>MRKFILSLSILLSALLVACSSRNHYGDTGSLAGLQAMADSKYTRAQKKQKMGKIREMALKETALSVGAQAGLAWRAKIIDEQLNKQARNLDAIYDFNSLVLEHNILPPVLLEGRNTLNLADAQSIRISDRTYKVAKQAHFITTPPTWRQYLWMDYVKPEAPNVTLLPKTKAEKEIWCIYTERGWKNGIDQANTILEENIARIKEDFGGMILYRKLLAMNMVSPPYVSHTDLGVTGDGSEIHIDDRVLRITALPELNVNSAEWRAAVAKDENALERFKNMEKLANQAKIVITNKSWQPIIAPVS[13x];>[26x]MNNNKIVIMFIFSALLAGCAGTMKFKKPPINNPSDDATIKLAEAAVSVSDSMLEMAKVEKVITPPSKDNTLTIPNAYNLQARASVDWSGPIEELTARIAKAAHFRFRVLGKSPSVPVLISISTKDESLAEILRDIDYQAGKKASIHVYPNSQVVELRYAKIYS;>[13x]MMKKYDQLCKYCLVIGLTFSMSCSIYAADQSDDAQQALQQLRMLQQKLSQNPSPDAQSGAGDGGDNAASDSTQQPNQSGQANAPAANQTATAGGDGQIISQDDAEVIDKKAFKDMTRNLYPLNPEQVVKLKQIYETSEYAKAATPGTPPKPTATSQFVNLSPGSTPPVIRLSQGFVSSLVFLDSTGAPWPIAAYDLGDPSSFNIQWDKTSNTLMIQATKLYNYGNLAVRLRGLNTPVMLTLIPGQKAVDYRVDLRVQGYGPNAKSMPTEEGIPPSANDLLLHVLEGVPPPGSRRLVVSGGDARAWLSNEKMYVRTNLTILSPGWLASMTSADGTHAYEMQKSPVLLVSWHGKVMQLKVEGL;>MRSLRTNYIYVLFKTTGLLFLLLLSACNRSGYIPENEVPKLPCRVDGACDATIIKMMTDLNKKGIKVASVGQNYLISIPASALFADQSPRLNWASYSLLNEIAAFLKQFRKIAITVTSYSSKYVSVKRERALTLARSRVVSEYLWSQGVDSRIIFTQGLGSDKPITSYTLGGDRSPNARVEITFRRAVA[13x];>[52x]AAAAAAAAAAAAAAAAAAAAAAAAAAAAAAAAAAAAAAAAAAAAAAAAAAAAAAAAAAAAAAAAAAAAAAAAAAAAAAAAAAAAAAAAAAAAAAAAAAAAAAAAAAAAAAAAAAAAAAAAAAAAAAAAAAAAAAAAAAAAAAAAAAAAAAAAAAAAAAAAAAAAAAAAAAAAAAAAAAAAAAAAAAAAAAAAAAAAAAAAAAAAAAAAAAAAAAAAAAAAAAAAAAAAAAAAAAAAAAAAAAAAAAAAAAAAAAAAAAAAAAAAAAAAAAAAAAAAAAAAAAAAAAAAAAAAAAAAAAAAAAAAAAAAAAAAAAAAAAAAAA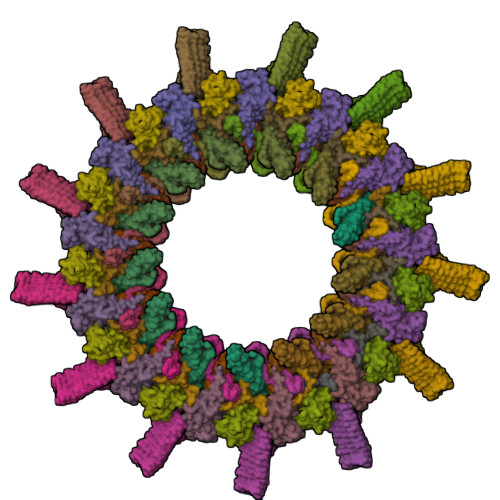AAAAAAAAMRNLMRCLIMIKSLIKGVDMSRKLAKTRILGYGLMICFLAGCFHPPYNNFQPDRRAVKRVGVDTGIGAVAGAIASGTASGTLIGAAAGGTVGLVASIYRDSKRKIIRDLQKQDIQYVEYGDTRTLIIPTDKYFMFSSPRLNEICYPGLNNVIRLLNFYPQSTIYVAGFTDNVGSRSHKRKLSQAQAETMMTFLWANGIAAKRLKAEGYGDKNAISDNAIIHGSAQNRRIEIQWFTSPAQPPQPQMAYVK> MSEEFGGQVVALVSVAETGVPGWGGLKAKARTTTRQPGV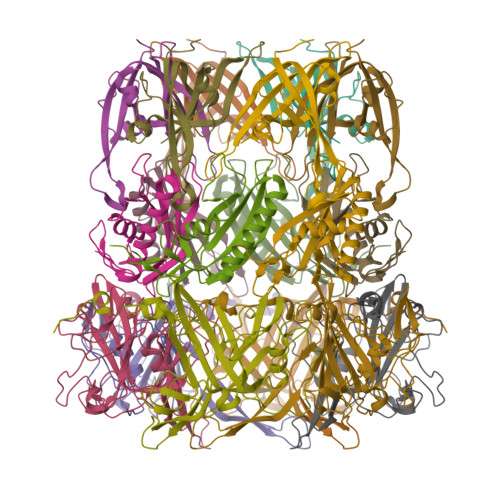HFRPASSTETPDGQTNVATEVWKLTAPPTAAVLAAKPGGELVYDGTEHPESLDLDSAAGRAATFRVDGPIMPKYDLAGQVHHVTIMCKRQAG;> MTMADLHDQDAPDEEDFVVCWMQPVMRTAVERDIDAELPFCEVTRIDGADDPEAGTDDPVIQLDFYALGAEAAKAAAKQGHRRMLFLFRNFPTVTLSDGTLADLDFGETLIKPSRMAFEHDQIVRYTARYQLGTSYVAVP;> MTQPLTGTTPAAGGYTTVDNRLQGGHRTGLIAVAFRDALGTSTNISPHNANGSVRWSPLAQDGQLRDDLFAHRLENGVWVENTNPNEGWYLAGAFGEGNGPSSRPSIDTDDQMIEQSNWPFESDITKQDEPFTFQALQNLYPAIQRLANNLPLSDANGNPLVELPGEADGFSQPVDAEKIGRQFLLYGIRKKEGRYLYEVDAYDLAYLNNKGERKFGKRGTAAELTFKPEPSGYFMAMVDGEYKPIIKHTFIGGPAWDALAGDGS2-(4-(3-HYDROXYPHENOXY)PHENYL)-1H-BENZO[D]IMIDAZOLE-5-CARBOXAMIDE | C20 H15 N3 O3 | 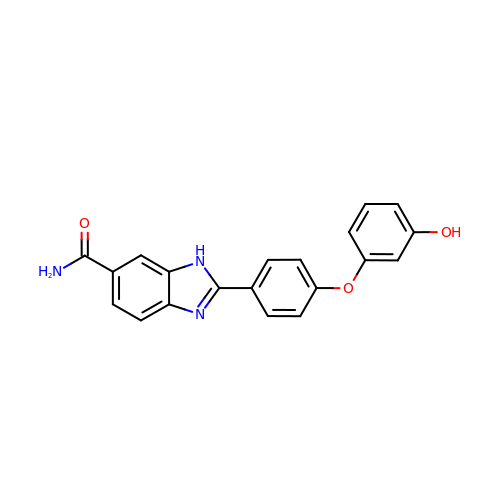PMCFOCQQFLSWEU-UHFFFAOYSA-N>MRGSHHHHHHGSMVLGKPQTDPTLEWFLSHCHIHKYPSKSTLIHQGEKAETLYYIVKGSVAVLIKDEEGKEMILSYLNQGDFIGELGLFEEGQERSAWVRAKTACEVAEISYKKFRQLIQVNPDILMRLSAQMARRLQVTSEKVGNLAFLDVTGRIAQTLLNLAKQPDAMTHPDGMQIKITRQEIGQIVGCSRETVGRILKMLEDQNLISAHGKTIVVYGTR[2x]

CAP is a 210-amino acid homodimeric transcription factor that binds cAMP generated by adenylyl cyclase in response to the phosphorylated form of Enzyme IIAGlc (phosphorylated in response to the phosphoenolpyruvate-carbohydrate phosphotransferase system). CAP regulates the transcription of over 100 genes required for the metabolism of diverse carbon sources through its binding to a specific promoter region and recruitment of RNA polymerase. Analysis of the two major ligand binding domains of the CAP homodimer demonstrated a homotropic negative allosteric interaction between cAMP binding sites and the absence of structural change within this domain. Negative allosteric cooperativity between cAMP binding sites in CAP occurs as a consequence of the protein-ligand contacts formed.

We used cAMP analogues to weaken CAP-cAMP interactions as an essential test of the predictions of the ENM. We selected Sp-cAMPS to remove the interaction between ligand and the Arg-82/Ser-83 pair, cIMP to remove the interaction between ligand, and the Thr-127/Ser-128 pair, and 2′-deoxy-cAMP to remove the interaction between ligand and the Gly-71/Glu-72 pair. We determined the crystal structure of CAP bound to Sp-cAMPS to confirm that the data were not explained by an unexpected change in the structure of CAP. Fig. 4a shows the x-ray crystal structure of CAP bound to Sp-cAMPS overlaid onto the structure of CAP bound to cAMP and demonstrates no significant difference in structure (root mean square deviation = 0.24 Å over 2177 atoms). We observe no significant conformational rearrangement of the ligand contacting residues, and the only inferred difference is the loss of a hydrogen bond between the phosphorothioate moiety of Sp-cAMPS and the hydroxyl group of Ser-83. The experimental data are therefore not explained by a change in protein conformation. The binding affinities of Sp-cAMPS and cIMP for CAP are therefore reduced in comparison to cAMP, as expected. Furthermore, K2/K1 for both analogues is also increased consistent with theoretical predictions. The computed and experimental data therefore demonstrate an unambiguous relationship between ligand interaction strength and allostery.> DYKDDDDKIAENEDALLRHLFQGYQKWVRPVLHSNDTIKVYFGLKISQLVDVDEKNQLMTTNVWLKQEWTDHKLRWNPDDYGGIHSIKVPSESLWLPDIVLFENADGRFEGSLMTKVIVKSNGTVVW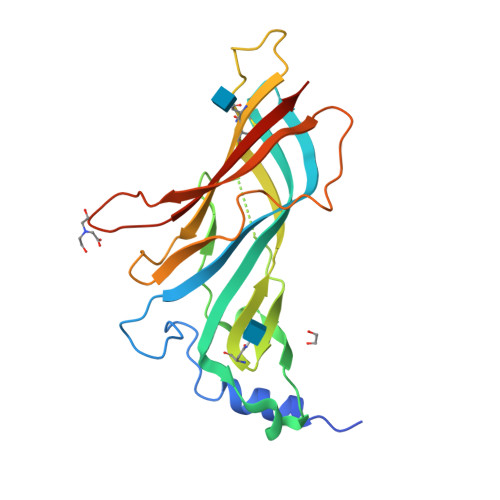TPPASYKSSCTMDVTYFPFDRQNCSMKFGSWTYDGTMVDLILINENVDRKDFFDNGEWEILNAKGMKGNRRDGVYSYPFITYSFVLRRHHHHHH>PPYTIVYFPVRGRCEAMRMLLADQGQSWKEEVVTIDTWMQGLLKPTALYGQLPKFEDGDLTLYQSNAILRHLGRSLGLYGKNQREAAQMDMVNDGVEDLRGKYVTLIYTNYENGKNDYVKALPGHLKPFETLLSQNQGGKAFIVGDQISFADYNLLDLLLIHQVLAPGCLDNFPLLSAYV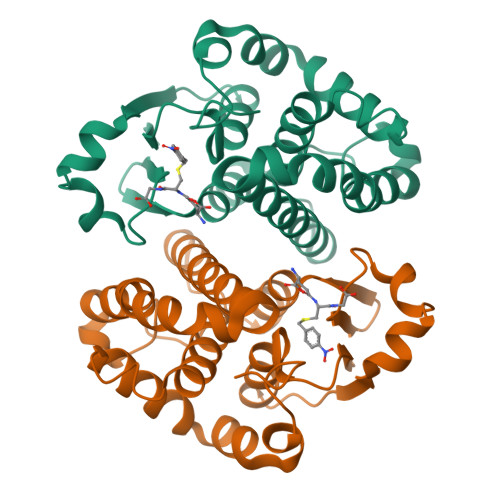ARLSARPKIKAFLSSPEHVNRPINGNGKQ[2x]>MGKVFLTNAFSINMLKEFPTTITIDKLDEEDFCLKLELRLEDGTLINAIGHDSTINLVNTLCGTQLQKNRVEVKMNEGDEAL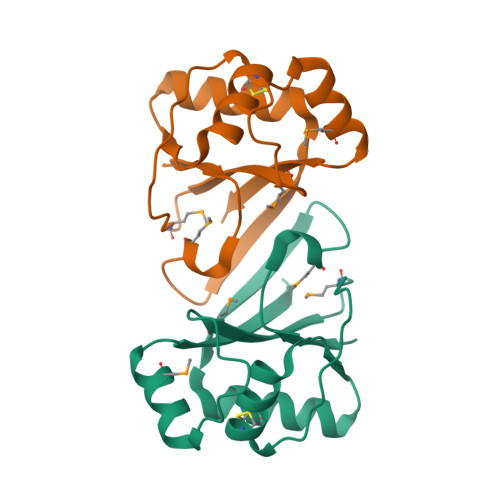IIMISQRLEEGKVLSDKEIKDMYRQGKISFYEVWHHHHHH[2x]>MARFFIDRPVFAWVISLLIVLAGVLAIRFLPVAQYPDIAPPVVNVSASYPGASAKVVEEAVTAIIEREMNGAPGLLYTKATSSTGQASLTLTFRQGVNADLAAVEVQNRLKIVESRLPESVRRDGIYVEKAADSIQLIVTLTSSSGRYDAMELGEIASSNVLQALRRVEGVGKVETWGAEYAMRIWPDPAKLTSMNLSASDLVNAVRRHNARLTVGDIGNLGVPDSAPISATVKVDDTLVTPEQFGEIPLRIRADGGAIRLRDVARVEFGQSEYGFVSRVNQMTATGLAVKMAPGSNAVATAKRIRATLDELSRYFPEGVSYNIPYDTSAFVEISIRKVVSTLLEAMLLVFAVMYLFMQNFRATLIPTLVVPVALLGTFTVMLGLGFSINVLTMFGMVLAIGILVDDAIIVVENVERLMAEEGLSPHDATVKAMRQISGAIVGITVVLVSVFVPMAFFSGAVGNIYRQFAVTLAVSIGFSAFLALSLTPALCATLLRPIDADHHEKRGFFGWFNRAFLRLTGRYRNAVAGILARPIRWMLVYALVIGVVALLFVRLPQAFLPEEDQGDFM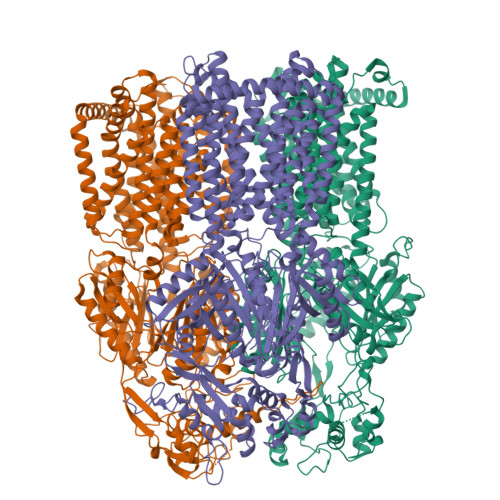IMVMQPEGTPMAETMANVGDVERYLAEHEPVAYAYAVGGFSLYGDGTSSAMIFATLKDWSERREASQHVGAIVERINQRFAGLPNRTVYAMNSPPLPDLGSTSGFDFRLQDRGGVGYEALVKARDQLLARAAEDPRLANVMFAGQGEAPQIRLDIDRRKAETLGVSMDEINTTLAVMFGSDYIGDFMHGSQVRKVVVQADGAKRLGIDDIGRLHVRNEQGEMVPLATFAKAAWTLGPPQLTRYNGYPSFNLEGQAAPGYSSGEAMQAMEQLMQGLPEGIAHEWSGQSFEERLSGAQAPALFALSVLIVFLALAALYESWSIPLAVILVVPLGVLGALLGVSLRGLPNDIYFKVGLITIIGLSAKNAILIIEVAKDHYQEGMSLLQATLEAARLRLRPIVMTSLAFGFGVVPLALSSGAGSGAQVAIGTGVLGGIVTATVLAVFLVPLFFLVVGRLFRLRKA[3x]>[5x]GASQFFKDNCNRTTASLVEGVELTKYIS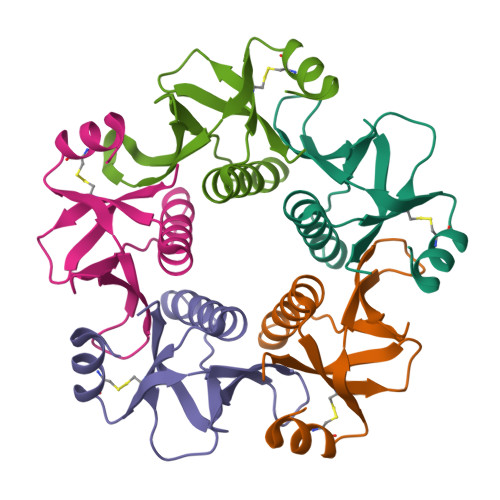DINNNTDGMYVVSSTGGVWRISRAKDYPDNVMTAEMRKIAMAAVLSGMRVNMCASPASSPNVIWAIELEAE>MNVLWIIALVGQLMRLVQGTATCAMYGNCGKKSVFGNELPCPVPRSFEPPVLSDETSKLLVEVCGEEWKEVRYACCTKDQVVALRDNLQKAQPLISSCPACLKNFNNLFCHFTCAADQGRFVNITKVEKSKEDKDIVAELDVFMNSSWASEFYDSCKNIKFSATNGYAMDLIGGGAKNYSQFLKFLGDAKPMLGGSPFQINYKYDLANEEKEWQEFNDEVYACDDAQYKCACSDCQESCPHLKPLVPR[4x]

In eukaryotes, integration of sterols into the vacuolar/lysosomal membrane is critically dependent on the Niemann–Pick type C (NPC) system. The system consists of an integral membrane protein, called NCR1 in yeast, and NPC2, a luminal soluble protein that transfers sterols to the N-terminal domain (NTD) of NCR1 before membrane integration. NCR1 and hNPC1 share the same structural fold: an N-terminal domain (NTD), a middle-luminal domain, and a C-terminal domain found on the luminal side of the vacuolar/lysosomal membrane. The current transport model for the NPC system postulates that NPC2 binds sterols in the lumen and loads them into the NTD, which transfers the sterol to a tunnel that is formed by the middle-luminal domain and C-terminal domain of hNPC1 and NCR1, respectively.

To study the substrate scope of NCR1, the NTD (residues 1–249 of NCR1) was purified and crystallized with either ergosterol or cholesterol: ergosterol-bound structure at 2.4 Å (Rfree 26%) and cholesterol-bound structure at 2.6 Å (Rfree 26%). Besides the sterol, the two structures show minimal differences between them (root mean square deviation of C-alpha atoms, RMSDCα, of 0.39 Å). Ergosterol and cholesterol are highly similar in their chemical structure, but the quality of the electron density maps allows for clear discernment between the two in the NTD binding pocket. Cholesterol lacks this double bond in the iso-octyl chain, making it more flexible, and this is observed as density that is discontinuous with the ring system. The hydroxyl group of cholesterol is closer to Q80, 2.8 Å away. The substrate binding pockets of the two structures are virtually identical, with both substrates positioned parallel to helix 2. Structurally, however, the substrate binding pocket of the NTD from yeast is less occluded, with 10.2 Å between K90 and I172, compared with 8.1 Å between the equivalent residues in the NTD of hNPC1. Even though the binding pocket of the NTD is less occluded, cholesterol seems to bind 1.0 Å deeper compared with the NTD from hNPC1. The clear density of an ion in a well-defined cation coordination site on the “back” of the NTD was identified. Because ZnSO4 was used in the crystallization solution, a zinc ion was modeled.>[16x]MNFIKDNSRALIQRMGMTVIKQIT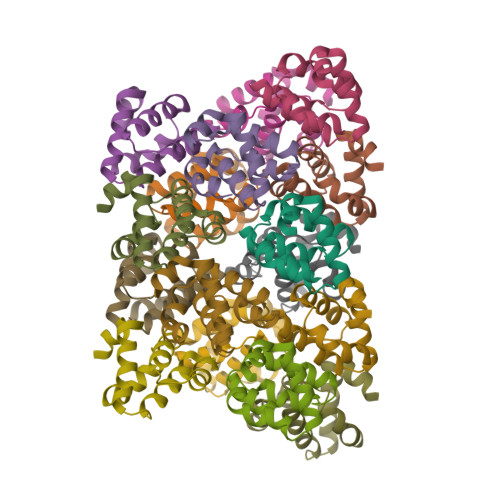DDLFVWNVLNREEVNIICCEKVEQDAARGIIHMILKKGSESCNLFLKSLKEWNYPLFQDLN>SNAMNSAALKSCLERENALVVEFLHALEAETEALMDRRAHESLQAAVQRKETLADDLAQLGAERDALLSGAGLASGPAGTDAAAAAHPELGPLWQALQANAAQARE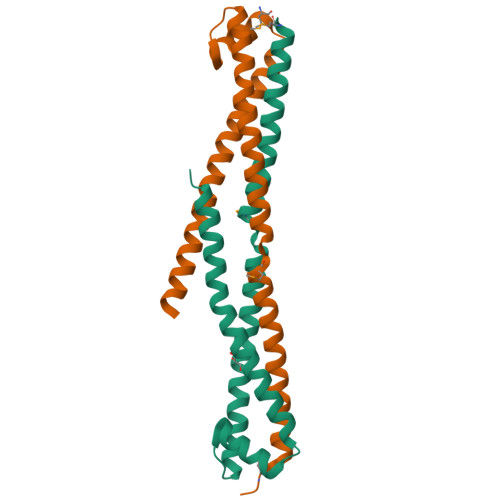HNQRNGTLIAVNLRHTQESLDALRQAAGTGAAATYDAQGRGKRGYSSA[2x]(furan-2-yl)acetic acid | C6 H6 O3 | 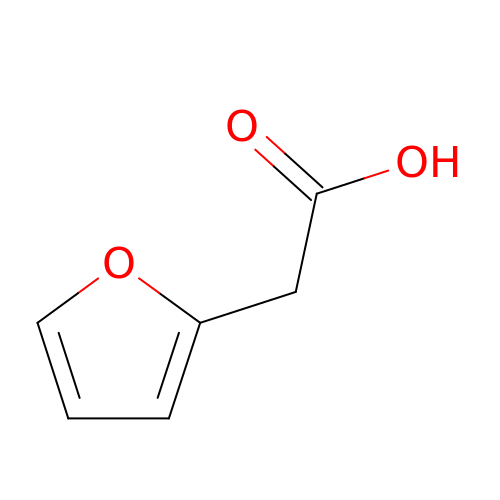VYSRZETUSAOIMP-UHFFFAOYSA-N> MKEFYLTVEQIGDSIFERYIDSNGRERTREVEYKPSLFAHCPESQATKYFDIYGKPCTRKLFANMRDASQWIKRMEDIGLEALGMDDFKLAYLSDTYNYEIKYDHTKIRVANFDIEVTSPDGFPEPSQAKHPIDAITHYDSIDDRFYVFDLLNSPYGNVEEWSIEIAAKLQEQGGDEVPSEIIDKIIYMPFDNEKELLMEYLNFWQQKTPVILTGWNVESFAIPYVYNRIKNIFGESTAKRLSPHRKTRVKVIENMYGSREIITLFGISVLDYIDLYKKFSFTNQPSYSLDYISEFELNVGKLKYDGPISKLRESNHQRYISYNIIAVYRVLQIDAKRQFINLSLDMGYYAKIQIQSVFSPIKTWDAIIFNSLKEQNKVIPQGRSHPVQPYPGAFVKEPIPNRYKYVMSFDLTSLYPSIIRQVNISPETIAGTFKVAPLHDYINAVAERPSDVYSCSPNGMMYYKDRDGVVPTEITKVFNQRKEHKGYMLAAQRNGEIIKEALH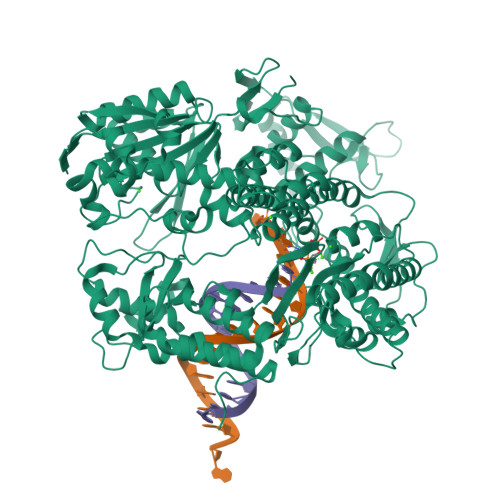NPNLSVDEPLDVDYRFDFSDEIKEKIKKLSAKSLNEMLFRAQRTEVAGMTAQINRKLLINSLAGALGNVWFRYYDLRNATAITTFGQMALQWIERKVNEYLNEVCGTEGEAFVLYGDTDSIYVSADKIIDKVGESKFRDTNHWVDFLDKFARERMEPAIDRGFREMCEYMNNKQHLMFMDREAIAGPPLGSKGIGGFWTGKKRYALNVWDMEGTRYAEPKLKIMGLETQKSSTPKAVQKALKECIRRMLQEGEESLQEYFKEFEKEFRQLNYISIASVSSANNIAKYDVGGFPGPKCPFHIRGILTYNRAIKGNIDAPQVVEGEKVYVLPLREGNPFGDKCIAWPSGTEITDLIKDDVLHWMDYTVLLEKTFIKPLEGFTSAAKLDYEKKA> MIKIAITKGRIQKQVTKLLENADYDVEPILNLGRELQIKTKDDLQIIFGKPNDVITFLEHGIVDIGFVGKDTLDENDFDDYYELLYLKIGQCIFALASYPDFSN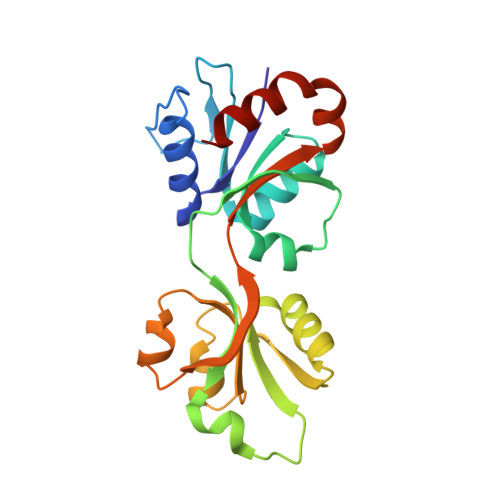KNFQRHKRIASKYPRVTKKYFAQKQEDIEIIKLEGSVELGPVVGLADAIVDIVETGNTLSANGLEVIEKISDISTRMIVNKSSFKFKKDKIIEMVERLEDAQTN> 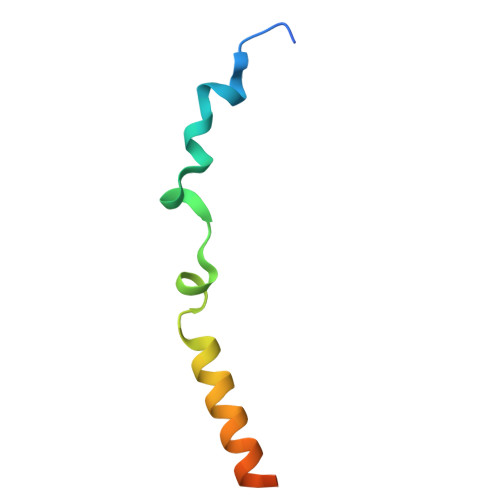MSSKIGFQWEKYEAWRYHPLLRFNKNTMFPGVGLGAAAFAVYYVVDTLSGDKSHH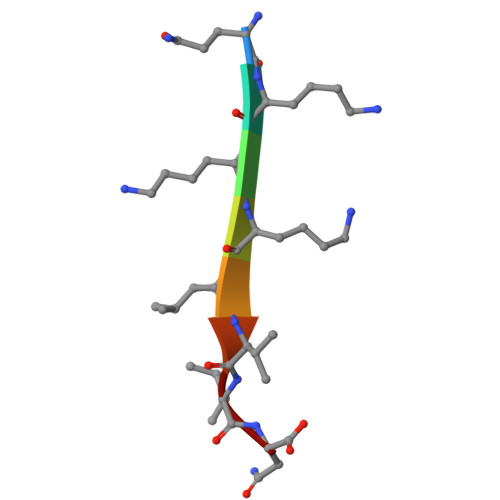> QKKKLVIN>GSHMMTGTIETTGNISAEKGGSIILQCHLSSTTAQVTQVNWEQQDQLLAICNADLGWHISPSFKDRVAPGPGLGLTLQSLTVNDTGEYFCIYHTYPDGTYTGRIFLEVLE[2x];>DVVVQAPTQVPGFLGDSVTLPCYLQVPNMEVTHVSQLTWARHGESGSMAVFHQTQGPSYSESKRL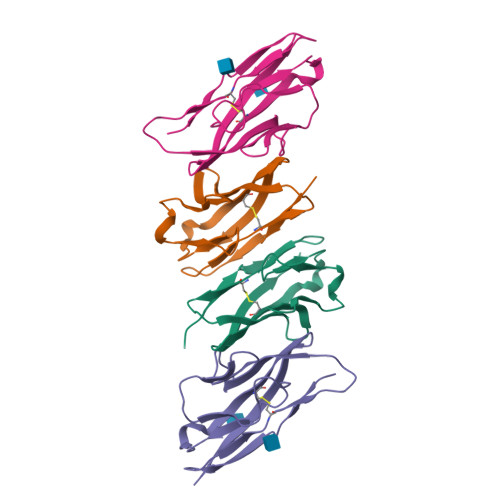EFVAARLGAELRNASLRMFGLRVEDEGNYTCLFVTFPQGSRSVDIWLRVLAKP[2x]>MMRRAYPEGPPPSYESVMQQAMAAAAAMQPPLEAPYVPPRYLAPTEGRNSIRYSELSPLYDTTRLYLVDNKSADIASLNYQNDHSNFLTTVVQNNDFTPTEASTQTINFDERSRWGGQLKTIMHTNMPNVNEYMFSNKFKARVMVSRKAPEGEFVTVNDGPVNDTYDHKEDILKYEWFEFILPEGNFSATMTIDLMNNAIIDNYLEIGRQNGVLESDIGVKFDTRNFRLGWDPETKLIMPGVYTYEAFHPDIVLLPGCGVDFTESRLSNLLGIRKRHPFQEGFKIMYEDLEGGNIPALLDVTAYEESKKDTTTARETTTLAVAEETSEDVDDDITRGDTYITELEKQKREAAAAEVSRKKELKIQPLEKDSKSRSYNVLEDKINTAYRSWYLSYNYGNPEKGIRSWTLLTTSDVTCGVEQVYWSLPDMMQDPVTFRSTRQVSNYPVVGAELMPVFSKSFYNEQAVYSQQLRQATSLTHVFNRFPENQILIRPPAPTITTVSENVPALTDHGTLPLRSSIRGVQRVTVTDARRRTCPYVYKALGIVAPRVLSSRTF[60x]

Adenovirus-derived nanoparticles (ADDomer) comprise 60 copies of adenovirus penton base protein (PBP). In the ADDomer, the PBP monomers spontaneously assembles to form a pentamer, and twelve pentamers organize into a dodecamer characterized by high stability and thermotolerance exceeding 50°C.16–18 The PBP monomer folds into two distinctive domains; the jelly-roll fold domain which is located in the core of the dodecamer and assumed to be responsible for multimerization, and a solvent-facing exterior domain, called the crown domain. The crown domain comprises two highly flexible regions, called variable loop (VL) and arginine-glycine-aspartic acid (RGD) motif-containing loop. To expand the scope of ADDomers for new applications, we engineered ADDobodies, representing PBP crown domain, genetically separated from PBP multimerization domain.

To test our concept that a selected ADDobody can be reconnected with a jelly-roll fold multimerization domain to yield ultra-high affinity ADDomer-based super-binders, we set out to graft ADDobody-AH0, derived from human adenovirus Ad3, onto the jelly-roll fold of the chimpanzee adenovirus serotype Y25 PBP to create a chimeric ADDomer, called Chimera, displaying 60 copies of AH0. This Chimera AH0 nanoparticle was produced using baculovirus/insect cell expression and purified by SEC and ion-exchange chromatography to homogeneity. After two-dimensional and three-dimensional (3D) classification and 3D refinement with applying icosahedral symmetry, we obtained a 2.2 Å resolution structure from 377,978 particles, resulting in the highest resolution for any ADDomer-derived nanoparticle structure to date. The overlay of the ADDomer Ad3 jelly-roll fold and the chimpanzee jelly-roll fold domain in our cryo-EM structure reveal a virtually identical fold, with an RMSD of 0.49 Å and differences only found in the N-terminal region of the jelly-roll. In the structure of the Chimera nanoparticle, the N-terminal regions comprising residues G47 to L59 of adjacent PBPs are observed to undergo strand swapping, stabilizing the interaction between pentons. In contrast, in our previous cryo-EM structure of the Ad3 ADDomer, we observed a hairpin conformation of the N-terminal residues, and the interaction between the N-termini was stabilized by hydrogen bonds between S61 and the main chain of E59. In our structure, the penton-penton interface of Chimera AH0, the N-terminus of the PBP forms an anti-parallel β-sheet with a PBP from an adjacent penton, involving residues 50–54 and residues 106−110. In addition, polar contacts are formed between R48 and S113, N49 and D61, and R52 and D110. Y53 can interact with N94 and Q105, further stabilizing the penton-penton interface. Chimera AH0 was passed at concentrations ranging from 0.325 to 1 nM over immobilized ADAH11, revealing strikingly low dissociation kinetics and an estimated avidity in the picomolar range (~200 pM).> A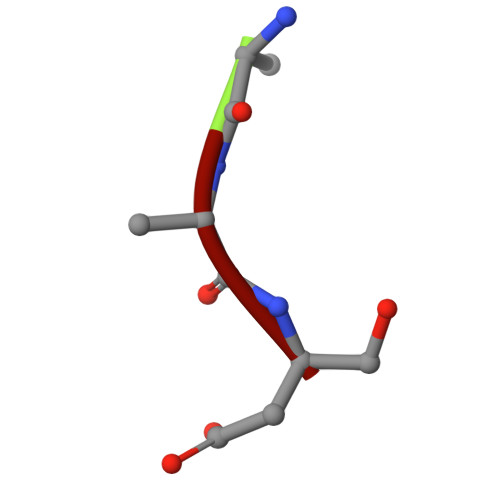AS D-2-AMINO-3-PHOSPHONO-PROPIONIC ACID | C3 H8 N O5 P | 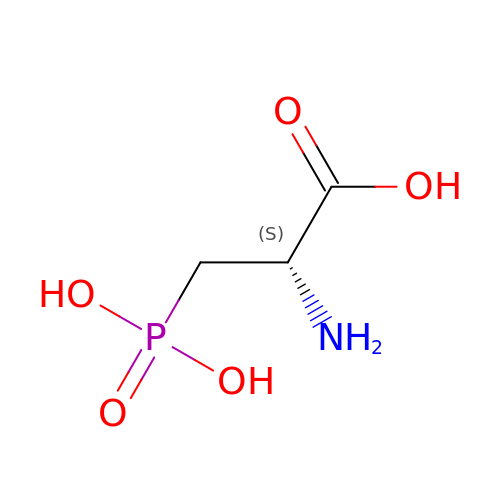LBTABPSJONFLPO-UWTATZPHSA-N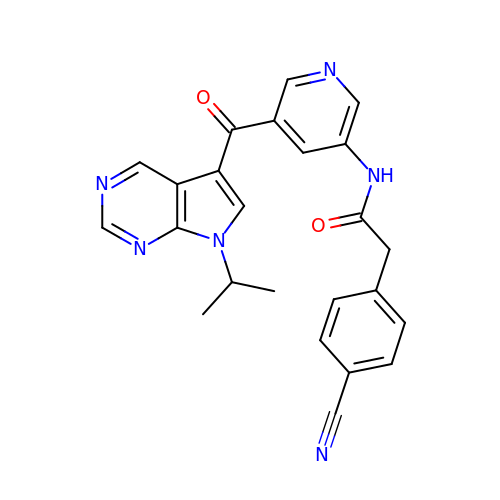2-(4-cyanophenyl)-N-{5-[7-(propan-2-yl)-7H-pyrrolo[2,3-d]pyrimidine-5-carbonyl]pyridin-3-yl}acetamide | C24 H20 N6 O2 | ZJYCGJNMKTVBQP-UHFFFAOYSA-N>[2x]MSISRRLFLRNAALSAALLSIKGQAIAKAAERTGIKDFYKDDFRIGTAVATATLTMKEKKPLLALIAREFNAITPENCMKWEPLKPQDKDWHWEAADKFVEFGEKHKMYIVGHNLVWHSQVPKEVFL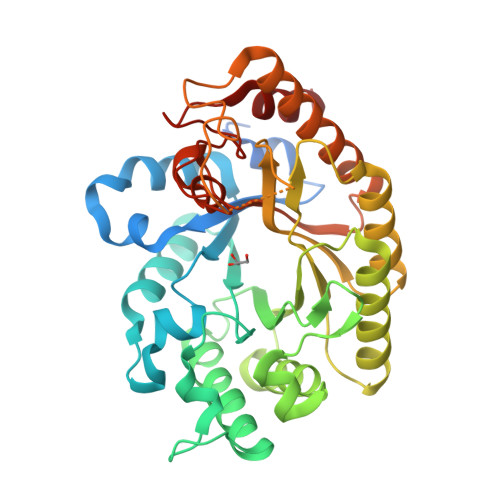NESGGTISKEALTAKMQDHIATLAGRYKGRIQAWDVVNEAVEDDGSWRKSPWYNIMGEDFIAKAFTMAHEVDPKAHLIYNDYNTESPIKRNFIVGMIKNFKKQGVPIHGVGMQEHLAIDGPSVDEIEKTLIALADAGVRAHITELDIDVLPSVWNLPTAEVSTRFEYKPERDPYIQGLPKDMEEKLAKRYEDIFKIYLKHRDKIERVTLWGTADNETWLNDFPIKGRTNYPLLFDRNQKPKPAYFRLLDLKK> NNLKEIEQEIEKVKNEKDAAVHAQEFENA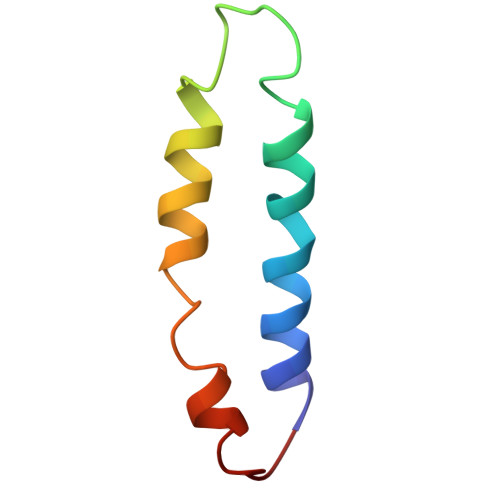ANLRDKQTKLEKQYEEAKNEWKNAQN>[2x]MRDPTQFEERHLKFLQQLGKGNFGSVEMCRYDPLQDNTGEVVAVKKLQHSTEEHLRDFEREIEILKSLQHDNIVKYKGVCYSAGRRNLKLIMEYLPYGSLRDYLQKHKERIDHIKLLQYTSQICKGMEYLGTKRYIHRDLATRNILVENENRVKIGDFGLTKVLPQDKEYYKVKEPGESPIFWYAPESLTESKFSVASDVWSFGVVLYELFTYIEK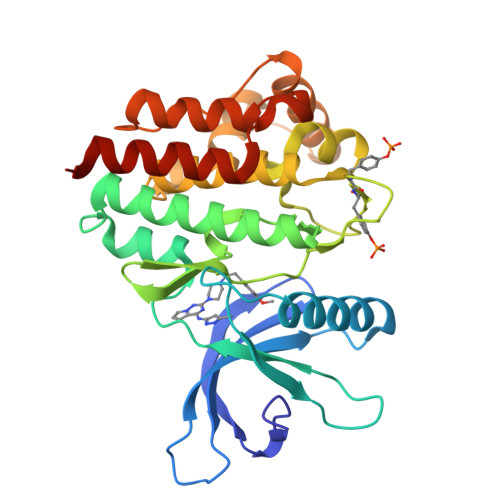SKSPPAEFMRMIGNDKQGQMIVFHLIELLKNNGRLPRPDGCPDEIYMIMTECWNNNVNQRPSFRDLALRVDQIRDNMAGHHHHHH> SDQALSFLKDFLAGGVAAAI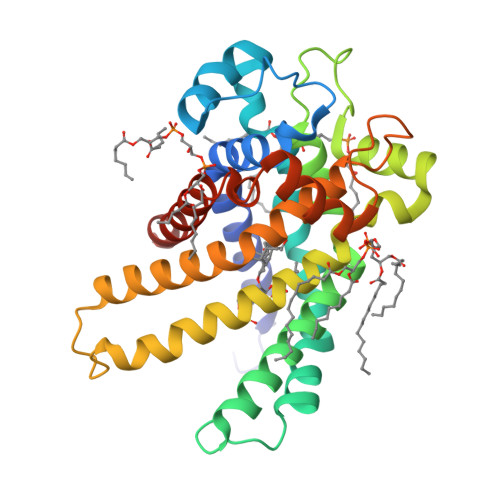SKTAVAPIERVKLLLQVQHASKQISAEKQYKGIIDCVVRIPKEQGFLSFWRGNLANVIRYFPTQALNFAFKDKYKQIFLGGVDRHKQFWRYFAGNLASGGAAGATSLCFVYPLDFARTRLAADVGKGAAQREFTGLGNCITKIFKSDGLRGLYQGFNVSVQGIIIYRAAYFGVYDTAKGMLPDPKNVHIIVSWMIAQTVTAVAGLVSYPFDTVRRRMMMQSGRKGADIMYTGTVDCWRKIAKDEGPKAFFKGAWSNVLRGMGGAFVLVLYDEIKKFV>MGQGPELHLASQFVNEACRALVFGGCVEKSSVSRNPEVPFESSAYRISASARGKELRLILSPLPGAQPQQEPLALVFRFGMSGSFQLVPREELPRHAHLRFYTAPPGPRLALCFVDIRRFGRWDLGGKWQPGRGPCVLQEYQQFRENVLRNLADKAFDRPICEALLDQRFFNGIGNYLRAEILYRLKIPPFEKARSVLEALQQHRPSPELTLSQKIRTKLQNPDLLELCHSVPKEVVQLGGRGYGSESGEEDFAAFRAWLRCYGMPGMSSLQDRHGRTIWFQGDPGPLAP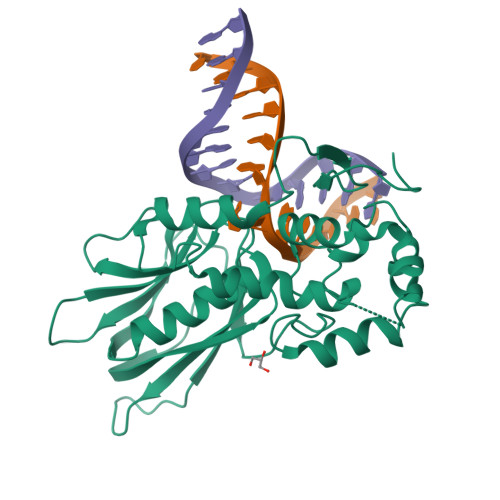KGRKS[3x]>MARKYFVAANWKCNGTLESIKSLTNSFNNLDFDPSKLDVVVFPVSVHYDHTRKLLQSKFSTGIQNVSKFGNGSYTGEVSAEIAKDLNIEYVIIGHFERRKYFHETDEDVREKLQASLKNNLKAVVCFGESLEQREQNKTIEVITKQVKAFVDLIDNFDNVILV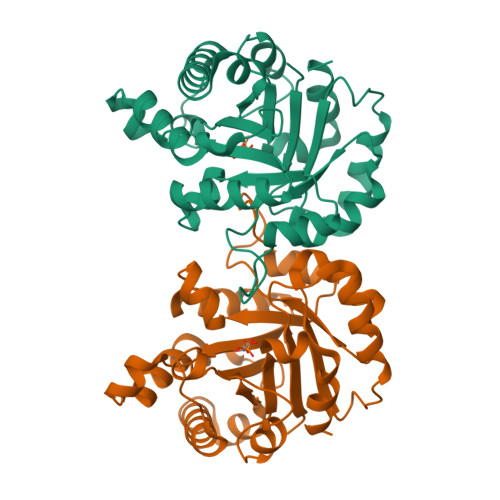YEPLWAIGTGKTATPEQAQLVHKEIRKIVKDTCGEKQANQIRILYGGSVNTENCSSLIQQEDIDGFLVGNASLKESFVDIIKSAM[2x]>[20x]MGDDARIAAIGDVDELNSQIGVLLAEPLPDDVRAALSAIQHDLFDLGGELCIPGHAAITEDHLLRLALWLVHYNGQLPPLEEFIL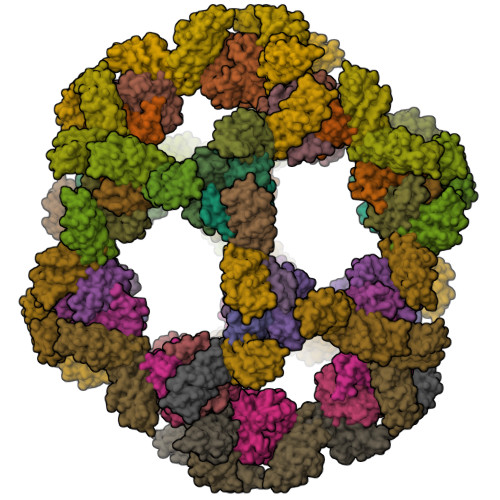PGGARGAALAHVCRTVCRRAERSIKALGASEPLNIAPAAYVNLLSDLLFVLARVLNRAAGGADVLWDRTRAH;>MILSAEQSFTLRHPHGQAAALAFVREPAAALAGVQRLRGLDSDGEQVWGELLVRVPLLGEVDLPFRSEIVRTPQGAELRPLTLTGERAWVAVSGQATAAEGGEMAFAFQFQAHLATPEAEGEGGAAFEVMVQAAAGVTLLLVAMALPQGLAAGLPPALEHHHHHH[20x]> GTGRSRLLEDFRNNRFPNLQLRDLIGHIVEFSQDQHGSRFIQQKLERATPAERQIVFNEILQAAYQLMTDVFGNYVIQKFFEFGSLDQKLALATRIRGHVLPLALQMYGCRVIQKALESISSDQQSEMVKELDGHVLKCVKDQNGNHVVQKCIECVQPQSLQFIIDAFKGQVFVLSTHPYGCRVIQRILEHCTAEQTLPILEELHQHTEQLVQDQYGNYVIQHVLEHGRPEDKSKIVSEIRGKVLALSQHKFASNVVEKCVTHASRAERALLIDEVCCQNDGPHSALYTMMKDQYANYVVQKMIDMAEPAQRKIIMHKIRPHIT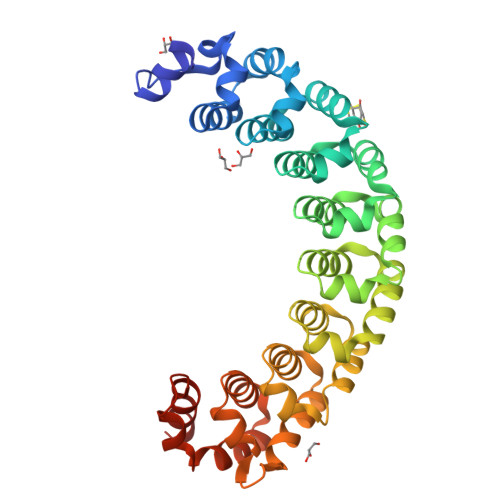TLRKYTYGKHILAKLEKYYLKNSPDLG>[2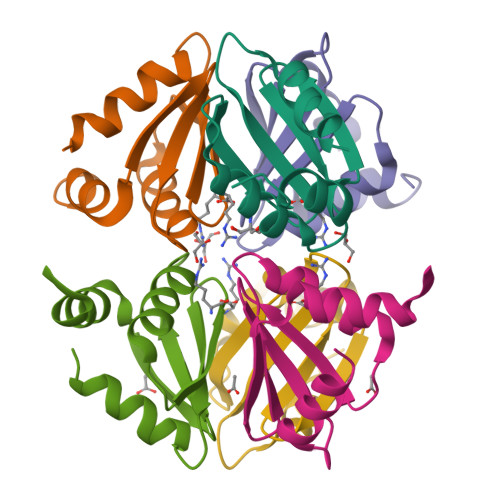x]VGTREKLRKMLDDLLVSVDHSGNIAVLRTPPGGAQFLASFIDRVGMEEVVGTIAGDDTVFVLARDPMTGQELGEFLSQRRSGN> MGYKEISLKYGKGAVDVKIDENMCTVLYPEDLPGVEDPMAEVSRSLKDPIGKAPLSDLVKGKKDVVILASDITRPSPSHILIPPITDELNRAGISDDSIKIVFGLGYHRKHTDDEKKTLVGEEVFNRIKCIDHDIDDCVYVGTTKRGTPVEVFREVYNADFIIATGNLELHYKAGYSGGHKALLPGVCSKNTIEKNHALMFSEGAMPGKIDGNPMREDIEEGGKLARVDFIVNAVLNSHKEIVKVVSGDPIKAHREGAKYIDKMYKRVIPEKADIVVASCGGYPKDINLYQAQKGLDNAQYSVKDGGTIILVAECREGLGEKLFSDWMVNSSSVDEPLKWIKEEFRLGAHKAAVICEVLKRADIYLISSFDRSLTEKIFFKYAKTPQDALDEAIKKYHDPKILVLPYANSTLPYVEEASWSHPQFEK

In this study, we investigated the substrate scope of several homologs of lactate racemase and discovered four new α-hydroxyacid racemases and one new α-hydroxyacid epimerase, thus uncovering a superfamily of NPN-dependent enzymes with various specificities and greatly expanding the number of known nickel enzymes, raising the number from 913 to 14. All of these reactions require the NPN cofactor, either added to the assay mix or previously bound to the protein, and lead to the inversion of a stereocenter at the C2 position of an α-hydroxyacid, suggesting the enzymes catalyze proton-coupled hydride transfer mechanisms as demonstrated for lactate racemization. The NPN cofactor, discovered in Lactobacillus plantarum LarA (hereafter referred to as just LarA), is synthesized from nicotinic acid adenine dinucleotide using the biosynthetic enzymes LarB, LarE, and LarC which catalyze carboxylation/hydrolysis, sulfur insertion, and nickel insertion reactions, respectively. Similarly, the catalytic residues (D72, H108, H174, and K298 in LarA) are also conserved in the Mar2 and GntE2 active sites, strongly confirming our hypothesis that these enzymes use the same catalytic mechanism as LarA.

To investigate the basis for substrate specificity of this family of enzymes, we crystallized Mar2 and compared it to the structure of LarA8. Although Mar2 was produced in L. lactis cells coexpressing the NPN-biosynthetic enzymes, the resulting structure lacked the NPN cofactor and substrate. A possible interpretation is that Mar2 is in an accessible state that is ready to receive the NPN cofactor. To better compare the Mar2 active site, which is poorly defined in the structure, we used I-Tasser19 to model Mar2 using the structure of LarA. We observed that the residues interacting with the NPN cofactor in LarA (R75, K184 and H200) have corresponding residues in Mar2 (R74, K181, and H197) and GntE2 (R41, K164, H180), suggesting that the binding mode for the cofactor is the same in these structures. The first region, hereafter named “loop”, is composed of the two residues just after a catalytic histidine (His174 in LarA); these residues are bulky and hydrophobic in LarA (F175 and F176), bulky and positively charged in Mar2 (Y172 and K173), and small polar and negatively charged for GntE2 (E155 and S156), consistent with the substrates they recognize. The second region is located in α-helix 11 (α11), in particular the residue before the catalytic K298 in LarA; this residue is V297 in LarA, a Q293 in Mar2, and G286 in GntE2. The last region potentially involved in substrate binding occurs in the first loop of α-helix 14 (α14), more specifically W358 in LarA, K351 in Mar2, and N348 in GntE2 that point in the direction of the substrate side chain.> ETGSPCKILKCNSEFWSATSGSHAPASDDTPEFCAALRSYALCTRRTARTCRGDLAYHSAVHGIEDLMSQHNCSKDGPT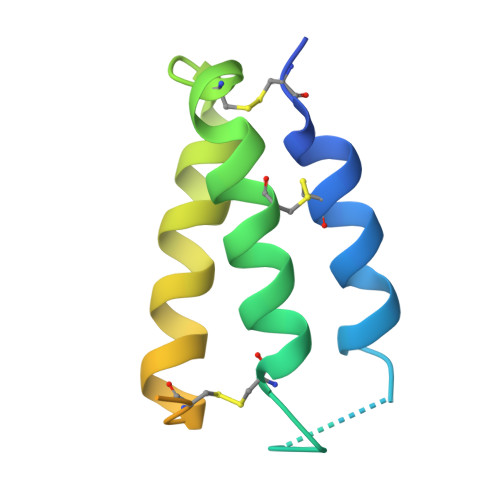SQPRLRTLPPAGDSQERSGTKHHHHHH> ESWVITEGRRLIPEIFQWSAVLSVCLGWPGAVYFFSK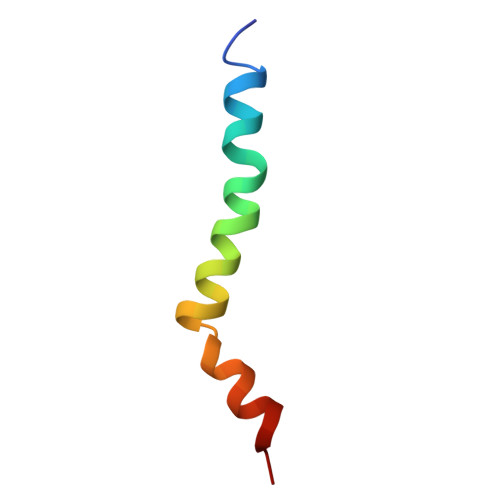A[(3S)-3-amino-4-hydroxy-4-oxo-butyl]-[[(2S,3S,4R,5R)-5-(6-aminopurin-9-yl)-3,4-dihydroxy-oxolan-2-yl]methyl]-methyl-selanium | 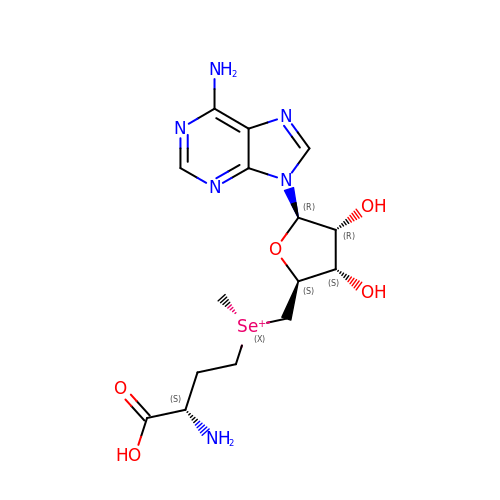C15 H23 N6 O5 Se | GGJFWMOVUFBSIN-FCKMPRQPSA-O>[5x]GPGSMWRETKLLLIDDNLDRSRDLAVILNFLGEDQLTCNSEDWREVAAGLSNSREALCVL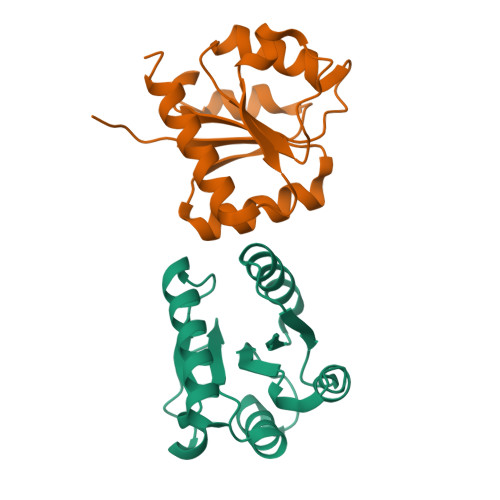LGSVESKGGAVELLKQLASWDEYLPILLIGEPAPADWPEELRRRVLASLEMPPSYNKLLDSLHRAQVYREMYDQARERGRSRE5-(4-fluorophenyl)-2,3-dihydroxy-N-[(E)-3-[(2R,3R,4R,5R)-4-hydroxy-3-methyl-5-[6-(propylamino)purin-9-yl]oxolan-2-yl]prop-2-enyl]benzamide 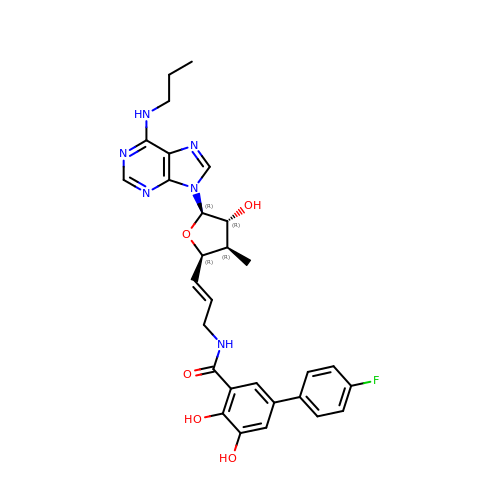| C29 H31 F N6 O5 | LOQQCXYJTZBLGY-SPGAZLGQSA-N>ALTCVMEGKDIEDWSCCPTPWTSFQSSCYFISTGMQSWTKSQKNCSVMGADLVVINTREEQDFIIQNLKRNSSYFLGLSDPGGRRHWQWVDQTPYNENVTFWHSGEPNNLDERCAIINFRSSEEWGWNDIHCHVPQKSICKMKKIYI[2x]

Blood dendritic cell antigen 2 (BDCA-2; also designated CLEC4C or CD303) is uniquely expressed on plasmacytoid dendritic cells. Sequence analysis reveals that BDCA-2 also contains a C-type CRD, despite the fact that it falls into a structurally distinct group of type 2 transmembrane receptors. Stimulation of BDCA-2 with antibodies initiates anti-inflammatory pathways through association with Syk kinase and adapter proteins such as Btk and BLNK, leading to stimulation of phospholipase C and a reduction in secretion of type 1 interferon. Binding, structural, and mutational analysis of the receptor suggest that it has a primary binding site for mannose, but that selectivity for galactose-terminated glycans is achieved through a secondary binding site.

To investigate the nature of the primary sugar-binding site in BDCA-2, crystallization of the CRD was attempted in the presence of Ca2+ and α-methyl mannoside to allow binding of the monosaccharide ligand. Crystals that diffracted to 1.65 Å were obtained starting from a solution containing 5 mm CaCl2 and 50 mm α-methyl mannoside. There are two copies of the molecule in the asymmetric unit. The overall fold of the main portion of the CRD is similar to mincle and other C-type CRDs, with the N-terminal extension forming an additional pair of β strands linked by a disulfide bond. The electron density maps indicated the presence of only one Ca2+ per monomer, bound by the five conserved residues noted in Fig. 1C, to create the primary sugar-binding site. α-Methyl mannoside is bound to this Ca2+ in both copies. In copy A, sugar is bound in two alternate orientations, with roughly the same occupancies, related by a 180° rotation that interchanges the positions of the 3- and 4-OH groups. These hydroxyl groups interact with the Ca2+ and its amino acid ligands by the network of coordination and hydrogen bonds that are characteristic of C-type CRDs. Although the search model contained three Ca2+, a striking difference between the crystal structure of BDCA-2 and the structure of mincle is the absence of the two accessory Ca2+-binding sites, one near the conserved site and one on the other side of the CRD, in BDCA-2. Notably, several of the acidic amino acid side chains that interact with these two additional Ca2+ in mincle have been substituted by basic amino acids. Measurement of the effect of Ca2+ concentration on 125I-Man-BSA binding to BDCA-2 confirmed that binding is Ca2+-dependent, but rather than being second order with respect to Ca2+ as was found for mincle, the binding is best fitted by first order dependence, consistent with the presence of the single Ca2+ site observed in the crystal structure.N-cyclopropyl-4-{[2-fluoro-4-(trifluoromethyl)phenyl]methyl}-3-methyl-1H-pyrrole-2-carboxamide 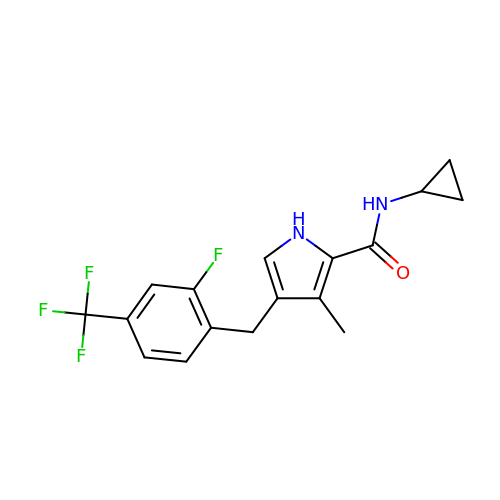| C17 H16 F4 N2 O | HLDSAPKKTAWHGH-UHFFFAOYSA-N>[3x]MSSKPKPIEIIGAPFSKGQPRGGVEKGPAALRKAGLVEKLKETEYNVRDHGDLAFVDVPNDSPFQIVKNPRSVGKANEQLAAVVAETQK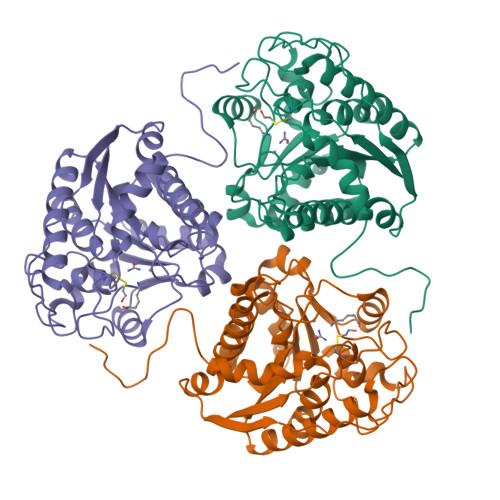NGTISVVLGGDHSMAIGSISGHARVHPDLCVIWVDAHTDINTPLTTSSGNLCGQPVAFLLKELKGKFPDVPGFSWVTPCISAKDIVYIGLRDVDPGEHYIIKTLGIKYFSMTEVDKLGIGKVMEETFSYLLGRKKRPIHLSFDVDGLDPVFTPATGTPVVGGLSYREGLYITEEIYKTGLLSGLDIMEVNPTLGKTPEEVTRTVNTAVALTLSCFGTKREGNHKPETDYLKPPK> KGSVYTAQSDVQVPENESIKLTCTYSGFSSPRVEWKFVQGSTTALVCYNSQITAPYADRVTFSSSGITFSSVTRKDNGEYTCMVSEEGGQNYGEVSIHLTVLVPPSKPTISVPSSVTIGNRAVLTCSEHDGSPPSEYSWFKDGISMLTADAKKT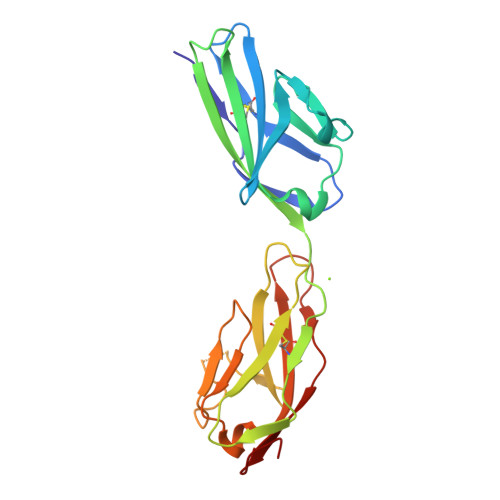RAFMNSSFTIDPKSGDLIFDPVTAFDSGEYYCQAQNGYGTAMRSEAAHMDAVELNVGG> GCGAAA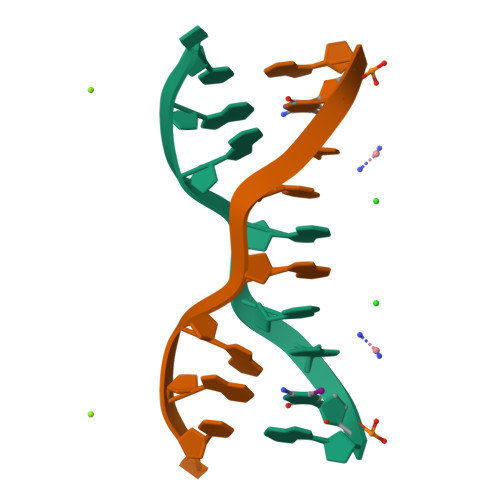GCT> MANMEARNVMSGTWGELWLDGNKVAEVKKFQAKMEFTKEDIIIAGQMGTDTKYMGYKGKGSITLYHVSSRMHKLIGEKIKRGSEPRFVAISKLNDPDSYGAERIAVKNIAFDDLTLADWEVGVKGEIEAPFTFTEYDFL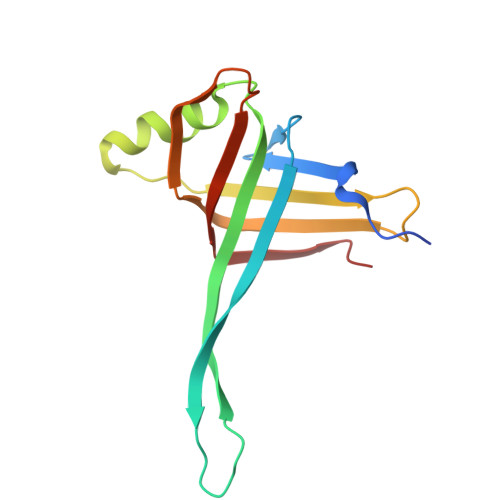DII>GSEAAGGEQRELLIQRLRAAVHYTTGALAQDVAEDKGVLFSKQTVAAISEITFRQAENFARDLEMFARHAKRSTITSEDVKLLARRSNSLLKYITQKSDELASSNME[2x];>[2x]GYEEREGGFRKETVERLLRLHFRDGRTRVNGDALLLMAELLKVFVREAAARAARQAQAEDLEKVDIEHVEKVLPQLL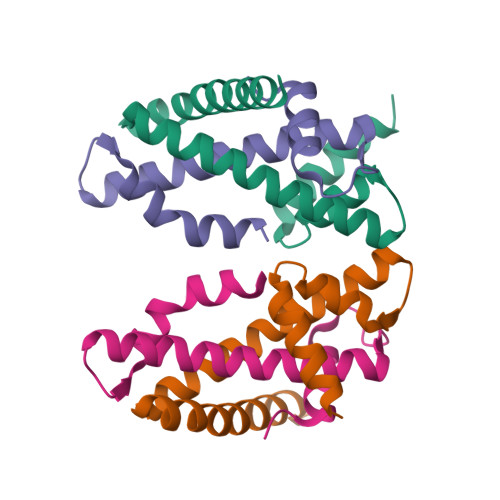LDFV>DWVIPPISCPENEKGEFPKNLVQIKSNRDKETKVFYSITGQGADKPPVGVFIIERETGWLKVTQPLDREAIAKYILYSHAVSSNGEAVADPMEIVITVTDQNDNRPEFTQEVFEGSVAEGAVPGTSVMKVSATDADDDVNTYNAAIAYTIVSQDPELPHKNMF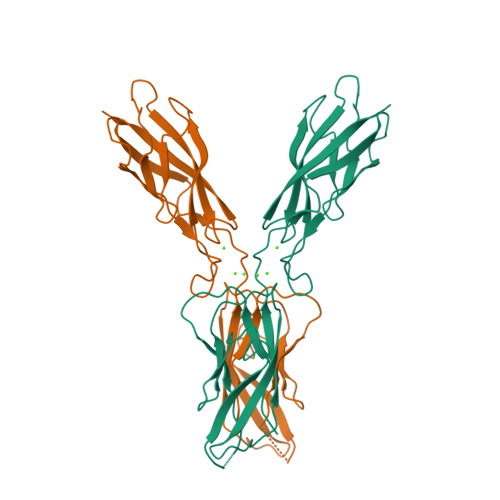TVNRDTGVISVLTSGLDRESYPTYTLVVQAADLQGEGLSTTAKAVITVKD[2x]OXONIC ACID | C4 H5 N3 O4 | 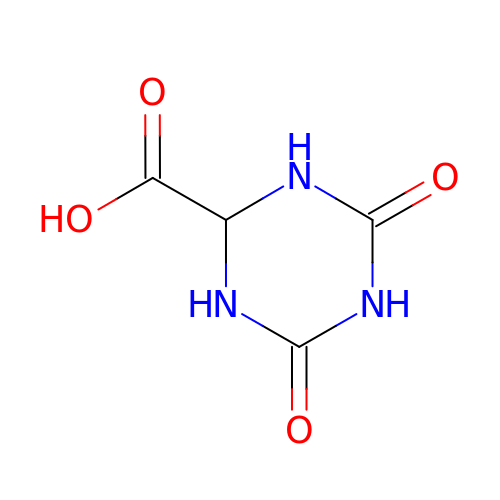IRFZLMWJJPULRF-UHFFFAOYSA-N Vertebrate type-IIa RPTPs comprise LAR, PTPσ and PTPδ, which share common domain architecture with a single transmembrane (TM) helix flanked by a large extracellular domain (ECD) and cytoplasmic tandem PTP domains: the membrane-proximal PTP domain (D1) is catalytically active, whereas the membrane-distal PTP domain (D2) is inactive. In mammals, presynaptic type-IIa RPTPs form trans-synaptic adhesion by specifically binding to their cognate postsynaptic organizers through their ECDs for inducing synaptic differentiation of neurons. To date, five different types of postsynaptic organizers for type-IIa RPTPs have been reported: interleukin-1 receptor (IL-1R) accessory protein (IL-1RAcP)7, IL-1RAcP-like-1 (IL1RAPL1)8, neurotrophin receptor tyrosine kinase C (TrkC), netrin-G ligand-3 (NGL-3)1011 and Slit- and Trk-like (Slitrk) family proteins. To elucidate the structural basis for decoding the ‘splice-insert signaling code' in the type-IIa RPTPs, we determined the crystal structures of PTPδ-ECD in complex with IL-1RAcP-ECD and IL1RAPL1-ECD.

The following Fn1 and Fn2 domains are aligned in a straight line, similarly to the isolated PTPδ Fn1-Fn2 structure, which we determined at 2.0 Å resolution.

>[2x]MALPKPPGTPVVTESTATSITLTWDSGNPEPVSYYIIQHKPKNSEEPYKEIDGIATTRYSVAGLSPYSDYEFRVVAVNNIGRGPASEPVLTQTSEQAPSSAPRDVQARMLSSTTILVQWKEPEEPNGQIQGYRVYYTMDPTQHVNNWMKHNVADSQITTIGNLVPQKTYSVKVLAFTSIGDGPLSSDIQVITLEHHHHHH> MSENWIDAAARDEVPEGDVIGINIVGKEIALYEVAGEIYATDNTCTHGAARMSDGFLEGREIECPLHQGRFDVCTGKA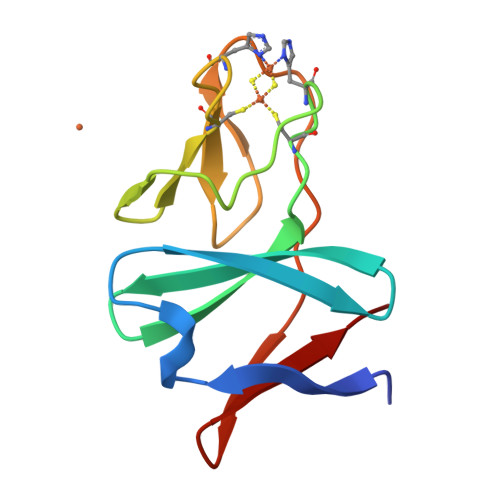LCTPLTQDIKTYPVKIENMRVMLKLD> MSAVKKQRIDLR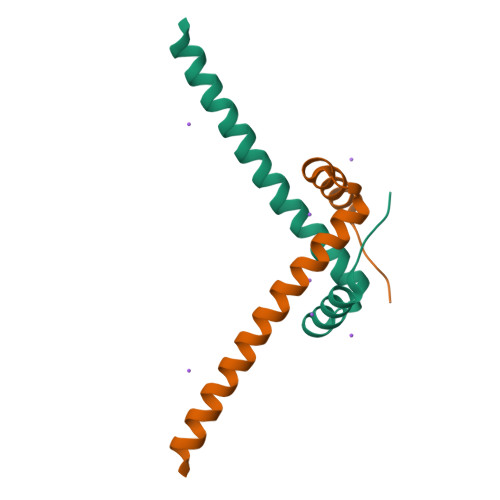LTDDDKSMIEEAAAISNQSVSQFMLNSASQRAAEVIEQHRRVILNEESWTRVMDALSNPPSPGEKLKRAAKRLQGM>MPQTSRVLLIIDDSPEDRELYRRYLLRDRDHSYTVLEAGLGRRGLELWQQHHPDAVLLDYRLPDLDGLEFLAKLQPPPQQPYLPVIMITGQGNEAIAVQAMKAGAQDYLVKEQITPEELHLAVNGAIETVHLRTQLHQRIERERVVSQITQKIHQTLDLEEILQTTVTEVRQFLQADRVFVYRFQPDFSGIVVLESVGDNCVPVIDAQVEDQYFVETRGEDYRQGRIQAVADIYTAGLTECHVNLLAQFHIRANLVVPILHADALWGLLVVNQCSAPRQWQPLEIDLLKELATQLGIALQQAEL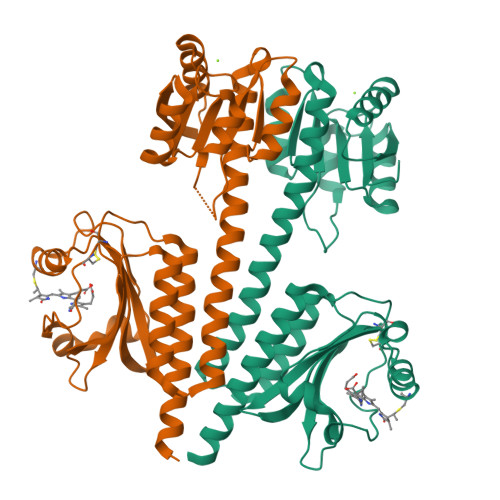YQQALEHHHHHH[2x]>[2x]MAKTIAYDEEARRGLERGLNALADAVKVTLGPKGRNVVLEKKWGAPTITNDGVSIAKEIELEDPYEKIGAELVKEVAKKTDDVAGDGTTTATVLAQALVREGLRNVAAGANPLGLKRGIEKAVEKVTETLLKGAKEVETKEQIAATAAISAGDQSIGDLIAEAMDKVGNEGVITVEESNTFGLQLELTEGMRFDKGYISGYFVTDPERQEAVLEDPYILLVSSKVSTVKDLLPLLEKVIGAGKPLLIIAEDVEGEALSTLVVNKI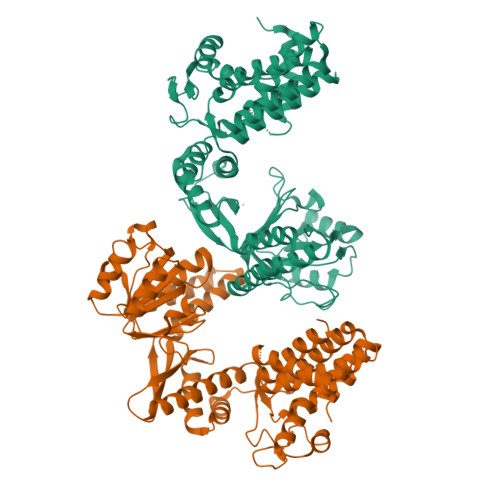RGTFKSVAVKAPGFGDRRKAMLQDMAILTGGQVISEEVGLTLENADLSLLGKARKVVVTKDETTIVEGAGDTDAIAGRVAQIRQEIENSDSDYDREKLQERLAKLAGGVAVIKAGAATEVELKERKHRIEDAVRNAKAAVEEGIVAGGGVTLLQAAPTLDELKLEGDEATGANIVKVALEAPLKQIAFNSGLEPGVVAEKVRNLPAGHGLNAQTGVYEDLLAAGVADPVKVTRSALQNAASIAGLFLTTEAVVADKPEKEKASVPGGGDMGGMDFHHHHHH> M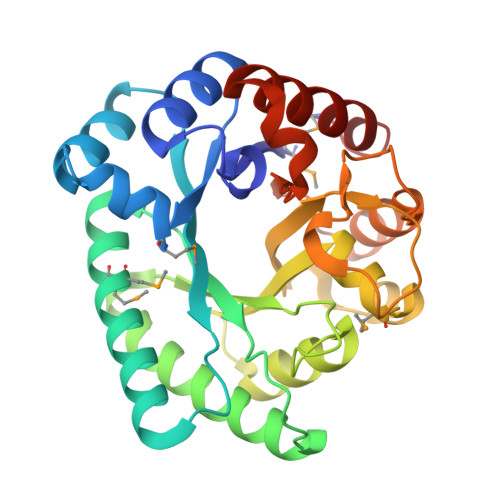KLCFNEATTLENSNLKLDLELCEKHGYDYIEIRTMDKLPEYLKDHSLDDLAEYFQTHHIKPLALNALVFFNNRDEKGHNEIITEFKGMMETCKTLGVKYVVAVPLVTEQKIVKEEIKKSSVDVLTELSDIAEPYGVKIALEFVGHPQCTVNTFEQAYEIVNTVNRDNVGLVLDSFHFHAMGSNIESLKQADGKKIFIYHIDDTEDFPIGFLTDEDRVWPGQGAIDLDAHLSALKEIGFSDVVSVELFRPEYYKLTAEEAIQTAKKTTVDVVSKYFSM>[2x]MLFKKDRKQETAYFSDSNGQQKNRIQLTNKHADVKKQLKMVRLGDAELYVLEQLQPLIQENIVNIVDAFYKNLDHESSLMDIINDHSSVDRLKQTLKRHIQEMFA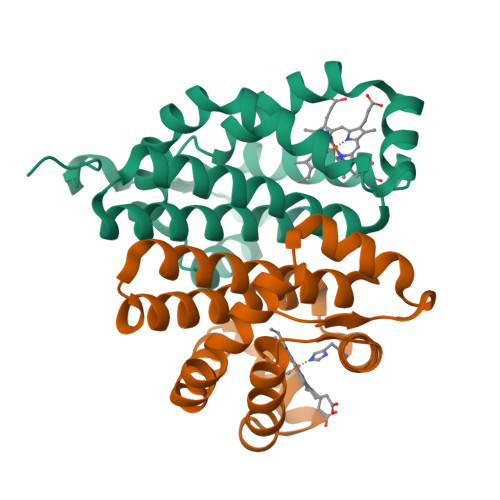GVIDDEFIEKRNRIASIHLRIGLLPKWYMGAFQELLLSMIDIYEASITNQQELLKAIKATTKILNLEQQLVLE> GPQDPYEINLMEELTLKGVTQYYAYVTERQKVHCLNTLF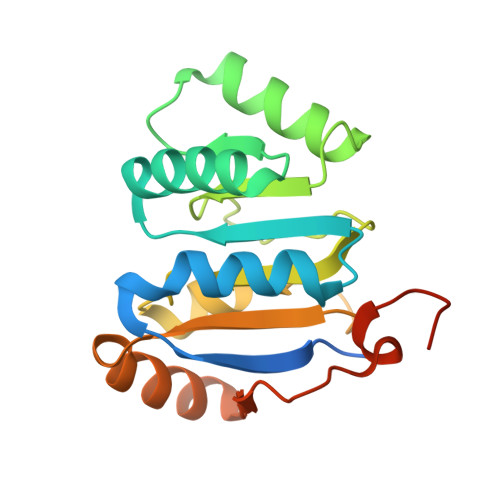SRLQINQSIIFCNSSQRVELLAKKISQLGYSCFYIHAKMRQEHRNRVFHDFRNGLCRNLVCTDLFTRGIDIQAVNVVINFDFPKLAETYLHRIGRSGRFGHLGLAINLITYDDRFNLKSIEEQLGTEIKPIPSNIDKSLYVAEYHSEPVEDEKP>SHVDPRIQGELEKLNQSTDDINRRETELEDARQKFRSVLVEATVKLD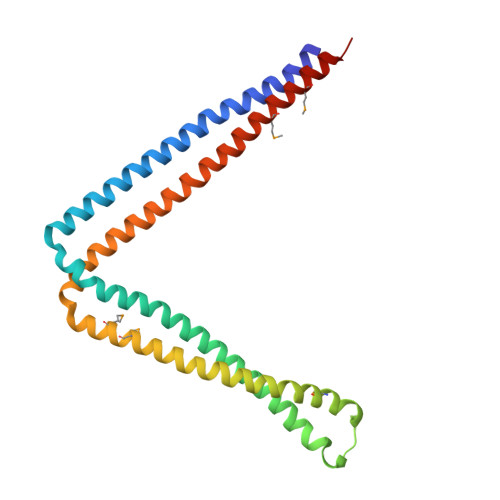ELVKKIGKAVEDSKPYWEARRVARQAQLEAQKATQDFQRATEVLRAAKETISLAEQRLLEDDKRQFDSAWQEMLNHATQRVAEAEQTKTRSELVHKETAARYNAAMGRMRQLEKKLKRAINKSKPYFELKAKYYVQLEQLKKTVDDLQAKLTLAKGEYKMALKNLEMISDEIHEAAASSAM[2x]> TDTTNSIKHVISPLARQTLQDRDLTRPVAGKRPIRLLPWLQVVKIGGRVMDRGADAILPLVEELRKLLPEHRLLILTGAGVRARH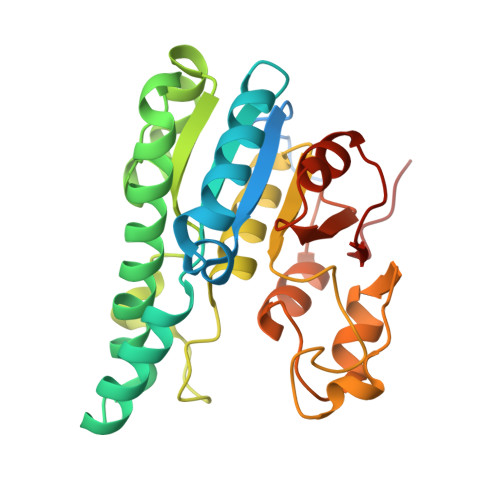VFSVGLDLGLPVGSLAPLAASEAGQNGHILAAMLASEGVSYVEHPTVADQLAIHLSATRAVVGSAFPPYHHHEFPGSRIPPHRADTGAFLLADAFGAAGLTIVENVDGIYTADPNGPDRGQARFLPETSATDLAKSEGPLPVDRALLDVMATARHIERVQVVNGLVPGRLTAALRGEHVGTLIRTGVRPA>MAPWKIEEVKTLKGLIKSKPVVAIVDMMDVPAPQLQEIRDKIRDKVKLRMSRNTLIIRALKEAAEELNNPKLAELANYVERGAAILVTDMNPFKLYKLLEENKSPAPVRGGQIAPCDIKVEKGSTGMPPGPFLGELKSVGIPAAIEKGKIAIKEDKVVVKKGEVVSPKLAAVLDRLGIKPIKVGLNILAVYEDGIIYTPDVLKVDEEK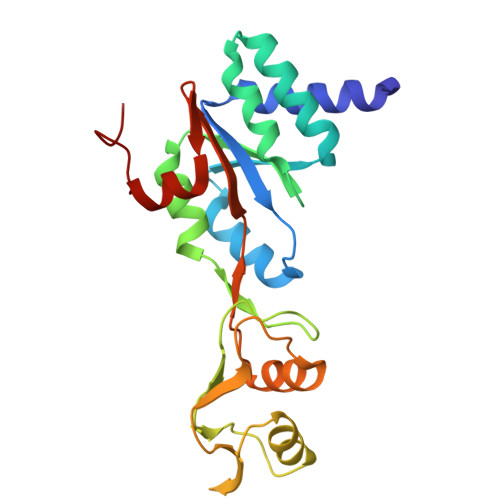LLADI[2x]The origin recognition complex (ORC), composed of Orc1–6, is a highly conserved heterohexameric complex, which plays a critical role in recognizing origin DNA and promoting helicase loading. Each of the Orc1–5 subunits bears an AAA+ or AAA+-like domain and an α-helical winged-helix domain (WHD). Among Orc1–5, Orc1, Orc4, and Orc5 each contains a functional AAA+ domain for nucleotide binding; in contrast, Orc2 and Orc3 only contain a RecA-like subdomain with no predicted ATPase activities. Away from DNA, metazoan ORC resides in an autoinhibited conformation with a closed and constricted central channel to preclude DNA binding.

In contrast, in State II (~60% particles, 4.8 Å), ORC2-WHD is relocated to an equivalent position of DmORC. In State II, ORC2-WHD retreats from the inner surface of the ORC ring, generating a hollow channel. Thereupon, a new interface is formed between the HTH motif of ORC2-WHD and the β-hairpin motif of ORC1-WHD. The limited resolution at this region did not allow an independent assignment of the side chains contributing to this interface. However, the involved motifs are highly conserved among the metazoan ORCs, a comparative analysis of the interface could be deduced from the crystal structure of DmORC. In DmORC, the equivalent residue of HsORC2-Phe524, that is Orc2-Phe566, is inserted into another hydrophobic cavity formed by five residues (Leu905, Ile892, Glu894, Lys903 and Glu851) from the β-hairpin of DmOrc1-WHD. The neighboring Arg563 and Glu564 of DmOrc2 interact with Asn907 and Arg889 of DmOrc1, respectively. The interaction between ORC1-WHD and ORC2-WHD induces the transition from State I to State II, which is likely the first step of ORC activation for origin DNA binding.

> MAHYPTRLKTRKTYSWVGRPLLDRKLHYQTYREMCVKTEGCSTEIHIQIGQFVLIEGDDDENPYVAKLLELFEDDSDPPPKKRARVQWFVRFCEVPACKRHLLGRKPGAQEIFWYDYPACDSNINAETIIGLVRVIPLAPKDVVPTNLKNEKTLFVKLSWNEKKFRPLSSELFAELNKPQESAAKCQKPVRAKSKSAESPSWTPAEHVAKRIESRHSASKSRQTPTHPLTPRARKRLELGNLGNPQMSQQTSCASLDSPGRIKRKVAFSEITSPSKRSQPDKLQTLSPALKAPEKTRETGLSYTEDDKKASPEHRIILRTRIAASKTIDIREERTLTPISGGQRSSVVPSVILKPENIKKRDAKEAKAQNEATSTPHRIRRKSSVLTMNRIRQQLRFLGNSKSDQEEKEILPAAEISDSSSDEEEASTPPLPRRAPRTVSRNLRSSLKSSLHTLTKVPKKSLKPRTPRCAAPQIRSRSLAAQEPASVLEEARLRLHVSAVPESLPCREQEFQDIYNFVESKLLDHTGGCMYISGVPGTGKTATVHEVIRCLQQAAQANDVPPFQYIEVNGMKLTEPHQVYVQILQKLTGQKATANHAAELLAKQFCTRGSPQETTVLLVDELDLLWTHKQDIMYNLFDWPTHKEARLVVLAIANTMDLPERIMMNRVSSRLGLTRMCFQPYTYSQLQQILRSRLKHLKAFEDDAIQLVARKVAALSGDARRCLDICRRATEICEFSQQKPDSPGLVTIAHSMEAVDEMFSSSYITAIKNSSVLEQSFLRAILAEFRRSGLEEATFQQIYSQHVALCRMEGLPYPTMSETMAVCSHLGSCRLLLVEPSRNDLLLRVRLNVSQDDVLYALKDE;> MSKPELKEDKMLEVHFVGDDDVLNHILDREGGAKLKKERAQLLVNPKKIIKKPEYDLEEDDQEVLKDQNYVEIMGRDVQESLKNGSATGGGNKVYSFQNRKHSEKMAKLASELAKTPQKSVSFSLKNDPEITINVPQSSKGHSASDKVQPKNNDKSEFLSTAPRSLRKRLIVPRSHSDSESEYSASNSEDDEGVAQEHEEDTNAVIFSQKIQAQNRVVSAPVGKETPSKRMKRDKTSDLVEEYFEAHSSSKVLTSDRTLQKLKRAKLDQQTLRNLLSKVSPSFSAELKQLNQQYEKLFHKWMLQLHLGFNIVLYGLGSKRDLLERFRTTMLQDSIHVVINGFFPGISVKSVLNSITEEVLDHMGTFRSILDQLDWIVNKFKEDSSLELFLLIHNLDSQMLRGEKSQQIIGQLSSLHNIYLIASIDHLNAPLMWDHAKQSLFNWLWYETTTYSPYTEETSYENSLLVKQSGSLPLSSLTHVLRSLTPNARGIFRLLIKYQLDNQDNPSYIGLSFQDFYQQCREAFLVNSDLTLRAQLTEFRDHKLIRTKKGTDGVEYLLIPVDNGTLTDFLEKEEEEA;> MATSSMSKGCFVFKPNSKKRKISLPIEDYFNKGKNEPEDSKLRFETYQLIWQQMKSENERLQEELNKNLFDNLIEFLQKSHSGFQKNSRDLGGQIKLREIPTAALVLGVNVTDHDLTFGSLTEALQNNVTPYVVSLQAKDCPDMKHFLQKLISQLMDCCVDIKSKEEESVHVTQRKTHYSMDSLSSWYMTVTQKTDPKMLSKKRTTSSQWQSPPVVVILKDMESFATKVLQDFIIISSQHLHEFPLILIFGIATSPIIIHRLLPHAVSSLLCIELFQSLSCKEHLTTVLDKLLLTTQFPFKINEKVLQVLTNIFLYHDFSVQNFIKGLQLSLLEHFYSQPLSVLCCNLPEAKRRINFLSNNQCENIRRLPSFRRYVEKQASEKQVALLTNERYLKEETQLLLENLHVYHMNYFLVLRCLHKFTSSLPKYPLGRQIRELYCTCLEKNIWDSEEYASVLQLLRMLAKDELMTILEKCFKVFKSYCENHLGSTAKRIEEFLAQFQSLDETKEEEDASGSQPKGLQKTDLYHLQKSLLEMKELRRSKKQTKFEVLRENVVNFIDCLVREYLLPPETQPLHEVVYFSAAHALREHLNAAPRIALHTALNNPYYYLKNEALKSEEGCIPNIAPDICIAYKLHLECSRLINLVDWSEAFATVVTAAEKMDANSATSEEMNEIIHARFIRAVSELELLGFIKPTKQKTDHVARLTWGGC;> MSSRKSKSNSLIHTECLSQVQRILRERFCRQSPHSNLFGVQVQYKHLSELLKRTALHGESNSVLIIGPRGSGKTMLINHALKELMEIEEVSENVLQVHLNGLLQINDKIALKEITRQLNLENVVGDKVFGSFAENLSFLLEALKKGDRTSSCPVIFILDEFDLFAHHKNQTLLYNLFDISQSAQTPIAVIGLTCRLDILELLEKRVKSRFSHRQIHLMNSFGFPQYVKIFKEQLSLPAEFPDKVFAEKWNENVQYLSEDRSVQEVLQKHFNISKNLRSLHMLLMLALNRVTASHPFMTAVDLMEASQLCSMDSKANIVHGLSVLEICLIIAMKHLNDIYEEEPFNFQMVYNEFQKFVQRKAHSVYNFEKPVVMKAFEHLQQLELIKPMERTSGNSQREYQLMKLLLDNTQIMNALQKYPNCPTDVRQWATSSLSWL;> MPHLENVVLCRESQVSILQSLFGERHHFSFPSIFIYGHTASGKTYVTQTLLKTLELPHVFVNCVECFTLRLLLEQILNKLNHLSSSEDGCSTEITCETFNDFVRLFKQVTTAENLKDQTVYIVLDKAEYLRDMEANLLPGFLRLQELADRNVTVLFLSEIVWEKFRPNTGCFEPFVLYFPDYSIGNLQKILSHDHPPEYSADFYAAYINILLGVFYTVCRDLKELRHLAVLNFPKYCEPVVKGEASERDTRKLWRNIEPHLKKAMQTVYLREISSSQWEKLQKDDTDPGQLKGLSAHTHVELPYYSKFILIAAYLASYNPARTDKRFFLKHHGKIKKTNFLKKHEKTSNHLLGPKPFPLDRLLAILYSIVDSRVAPTANIFSQITSLVTLQLLTLVGHDDQLDGPKYKCTVSLDFIRAIARTVNFDIIKYLYDFL N,N-diethyl-N~2~-(3-phenylpropanoyl)-L-asparaginyl-O-methyl-N-[(naphthalen-1-yl)methyl]-L-serinamide 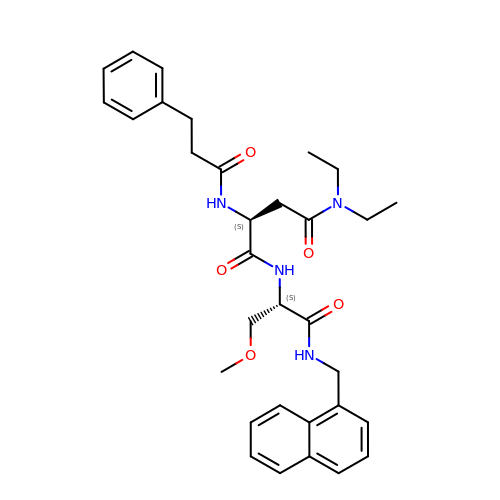| C32 H40 N4 O5 | VBXXQNRGFBZKES-NSOVKSMOSA-N>[2x]MYDLLVIGAGPGGYVAAIRAAQLGMKVGVVEKEKALGGTCLRVGCIPSKALLETTERIYEAKKGLLGAKVKGVELDLPALMAHKDKVVQANTQGVEFLFKKNGIARHQGTARFLSERKVLVEETGEELEARYILIATGSAPLIPPWAQVDYERVVTSTEALSFPEVPKRLIVVGGGVIGLELGVVWHRLGAEVIVLEYMDRILPTMDLEV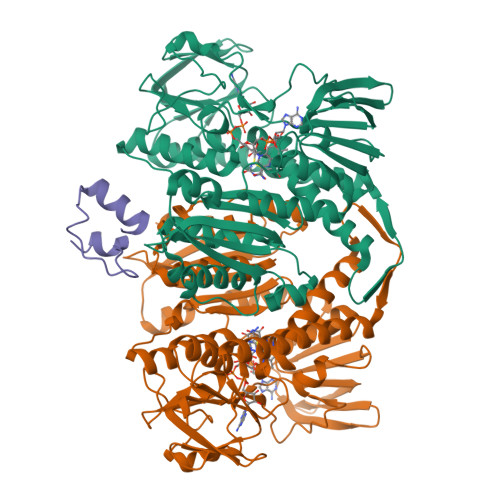SRAAERVFKKQGLTIRTGVRVTAVVPEAKGARVELEGGEVLEADRVLVAVGRRPYTEGLSLENAGLSTDERGRIPVDEHLRTRVPHIYAIGDVVRGPMLAHKASEEGIAAVEHMVRGFGHVDYQAIPSVVYTHPEIAAVGYTEEELKAQGIPYKVGKFPYSASGRARAMGETEGFIKVLAHAKTDRILGVHGIGARVGDVLAEAALALFFKASAEDLGRAPHAHPSLSEILKEAALAAWERPIHL;> LAMPAAERLMQEKGVSPAEVQGTGLGGRILKEDVMRHLEE>MMQN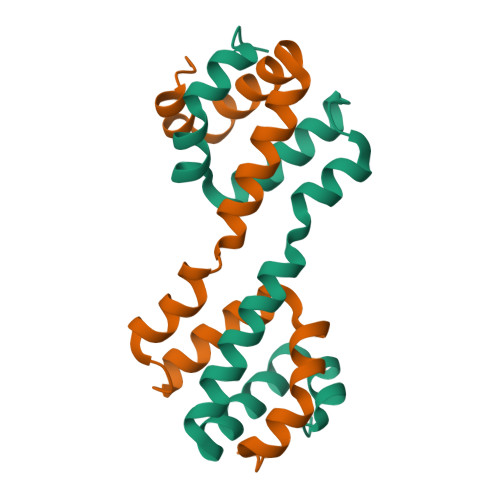FGAQEMRKGRLAFVRLSKLETLQNLIDKMLAERVFNKGEAADILESNDIRADIARALIDSVTKKGDVACSLFAGAIARQDVVLADAMGISQVLEHHHHHH[4x]>MGHHHHHHSHMSKESVTVAGIDCGTNSIRLKIARVDADGMHEVVPRILRVIRLGQDVDKTHRFADEALERAYVAAREFAGVIAEHPIDGLRFVATSATRDAENREEFEDEIERILGVRPEVIPGTEEADLSFLGATSVVNRDDLPAPYLVVDLGGGSTELVIGGDGVSAPTTQVQGAFSMNIGSVRMTERHLTNDPPTQTQIDEAVADVDEHIDEAFRTVDAGKARTIIGVSGTVTTMTAL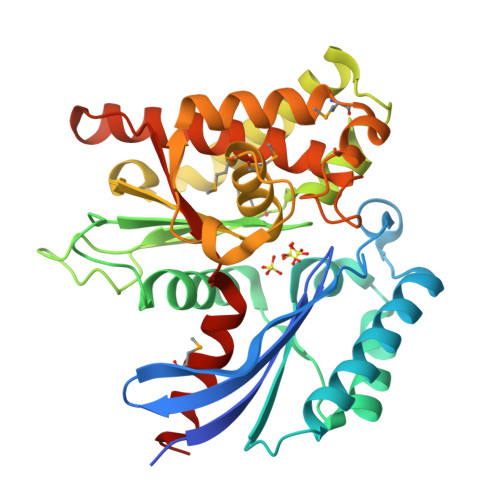AMGLKEYDHTVVDGHRLSFEDAYAVDDKFLRMTRAERREYKTIHPGRIDVVGGGAVVWSRVLARVSEAAKADHGEAIDSFVASEHGLLDGIVLDYGRRLLAQ[5x]> MENTENSVDSKSIKNLEPKIIHGSESMDSGISLDNSYKMDYPEMGLCIIINNKNFHKSTGMTSRSGTDVDAANLRETFRNLKYEVRNKNDLTREEIVELMRDVSKEDHSKRSS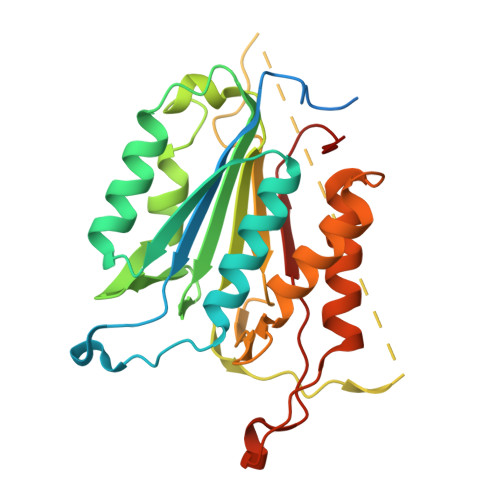FVCVLLSHGEEGIIFGTNGPVDLKKITNFFRGDRCRSLTGKPKLFIIQACRGTELDCGIETDSGVDDDMACHKIPVEADFLYAYSTAPGYYSWRNSKDGSWFIQSLCAMLKQYADKLEFMHILTRVNRKVATEFESFSFDATFHAKKQIPCIHSMLTKELYFYH>GSANDSPAKSLVDIDLSSLRDPAGIFELVEVVGNGTYGQVYKGRHVKTGQLAAIKVMDVTEDEEEEIKLEINMLKKYSHHRNIATYYGAFIKKSPPGHDDQLWLVMEFCGAGSITDLVKNTKGNTLKEDWIAYISREILRGLAHLHIHHVIHRDIKGQNVLLTENAEVKLVDFGVSAQLDRTVGRRNTFIGTPYWMAPEVIACDENPDATYDYRSDLWSCGITAIEMAEGAPPLCDMHPMRALFLIPRNPPPRLKSKKWSKKFFSFIEGCL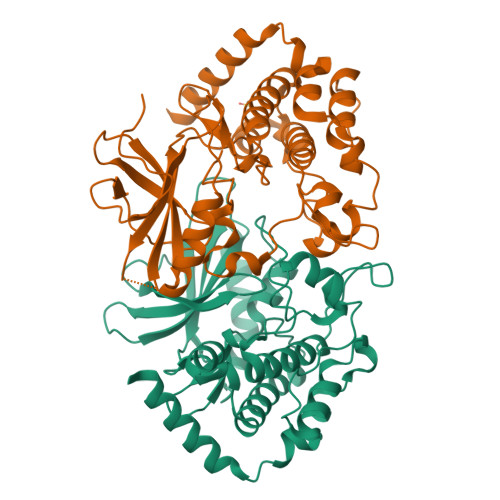VKNYMQRPSTEQLLKHPFIRDQPNERQVRIQLKDHIDRTRKKRGEKDETEYEYSGSEEGNS[2x]> MALAKRIIAALIVKDGRVVKGSNFENLRDSGDPVELGKFYSEIGIDELSFWDITASVEKRKTMLELVEKVAEQIDIPFTVGGGIHDFETASELILRGADKVEINTAAVENPSLITQIAQTFGSQAVVVYIAAKRVDGEFMVFTYSGKKNTGILLRDWVVEVEKRGAGEIVLGSIDRLGTKSGYDTEMIRFVRPLTTLPIIAHGGAGKMEHFLEAFLAGADAAKANSVLHFREIDVRELKEYLKKHGVNVRLEGLGSLEHHHH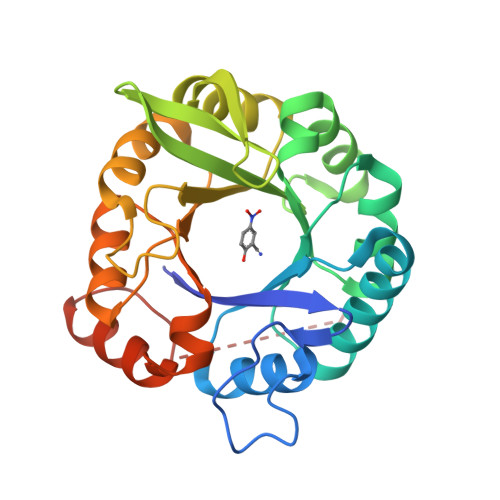HH Type III secretion systems (T3SSs) are membrane-embedded nanomachines that export dedicated proteins from the bacterial cytoplasm. FliD and FliC are found in complex with their dedicated chaperones FliT and FliS, respectively, in the cytoplasm. Here we report the structures of the ternary complexes among the FliD and FliC flagellar proteins, their cognate chaperones FliT and FliS, and the export gate protein FlhAC. FlhAC folds in a clamp-like structure with four discrete subdomains (d1 through d4).

The globular cytoplasmic domain of Salmonella enterica serovar Typhimurium FlhA (FlhAC) encompasses residues 362–692 (36.4 kDa) and is tethered to the transmembrane domain via a linker (residues 328–362). We determined the crystal structure of FlhAC at 1.9 Å resolution, which shows high similarity to a previously reported structure solved at 2.8 Å resolution of a longer FlhAC construct that includes the linker (FlhAC−link)26. Multiangle light scattering (MALS) data showed that FlhAC is monomeric in solution whereas the linker in FlhAC−link promotes a dimeric state that, based on the crystal structure, is mediated almost exclusively by electrostatic contacts. Indeed, FlhAC oligomerization is very sensitive to the salt concentration in solution. Structural comparison of FlhAC and FlhAC−link shows that the linker does not alter the three-dimensional fold of the protein. The cleft is hydrophobic and is lined by aliphatic and aromatic residues, as well as several Thr residues. The binding cleft is the most conserved surface in FlhAC highlighting the importance of this region to the function of FlhA.

> QGGGEDSLGMEVGYRLIPMVDFQQDGELLGRIRSIRKKFAQDMGFLPPVVHIRDNMDLQPARYRILMKGVEIGSGDAYPGRWLAINPGTAAGTLPGEKTVDPAFGLDAIWIESALKEQAQIQGFTVVEASTVVATHLNHLIGQFSAELFGRQEAQQLLDRVSQEMPKLTEDLVPGVVTLTTLHKVLQNLLAEKVPIRDMRTILETLAEHAPLQSDPHELTAVVRVALGRAITQQWFPGNEEVQVIGLDTALERLLLQALQGGGGLEPGLADRLLAQTQEALSRQEMLGAPPVLLVNHALRPLLSRFLRRSLPQLVVLSNLELSDNRHIRMTATIGGK> HHHHHHDYKDDDDKADPVPTSKPTPTGKGCHIGRFKSLSPQELASFKKARDALEESLKLKNWSCSSPVFPGNWDLRLLQVRERPVALEAELALTLKVLEAAAGPALEDVLDQPLHTLHHILSQLQACIQPQPTAGPRPRGRLHHWLHRLQEAPKKESAGCLEASVTFNLFRLLTRDLKYVADGNLCLRTSTHPEST;> PGRPRLAPPQNVTLLSQNFSVYLTWLPGLGNPQDVTYFVAYQSSPTRRRWREVEECAGTKELLCSMMCLKKQDLYNKFKGRVRTVS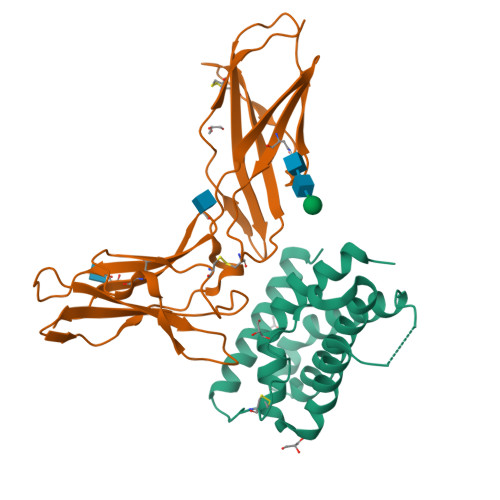PSSKSPWVESEYLDYLFEVEPAPPVLVLTQTEEILSANATYQLPPCMPPLDLKYEVAFWKEGAGNKTLFPVTPHGQPVQITLQPAASEHHCLSARTIYTFSVPKYSKFSKPTCFLLEVPEANASGSSGGSSGTSHHHHHH>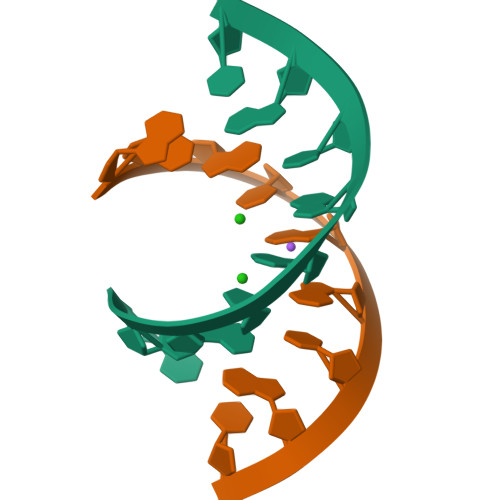[2x]AUGUGGCAU>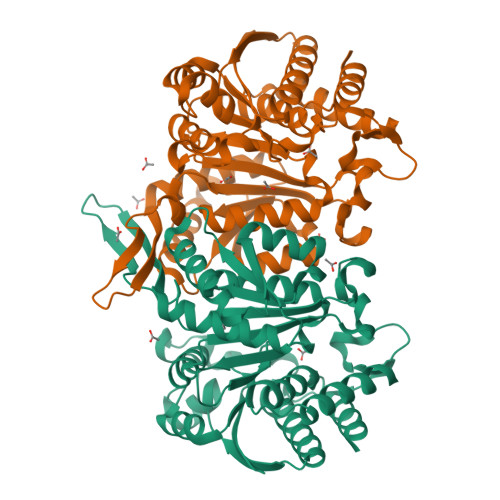MAAALQTNIRTVKVPATFRAVSKQSLAPFRVRCAVASPGKKRYTITLLPGDGIGPEVVSIAKNVLQQAGSLEGVEFNFREMPIGGAALDLVGVPLPEETISAAKESDAVLLGAIGGYKWDNNEKHLRPEKGLLQIRAALKVFANLRPATVLPQLVDASTLKREVAEGVDLMVVRELTGGIYFGEPRGIKTNENGEEVGFNTEVYAAHEIDRIARVAFETARKRRGKLCSVDKANVLEASILWRKRVTALASEYPDVELSHMYVDNAAMQLVRDPKQFDTIVTNNIFGDILSDEASMITGSIGMLPSASLSDSGPGLFEPIHGSAPDIAGQDKANPLATILSAAMLLKYGLGEEKAAKRIEDAVLVALNNGFRTGDIYSAGTKLVGCKEMGEEVLKSVDSQVPASV[4x]> GHMQGQIIHHRNFQSQFDTTGNTLYNNAWVCSLNVIKSRDGNNYSALEDITSDNQAFNNILEGIDIIECENLLKEMNVQKIPESSLFTNIKEALQAEVFNST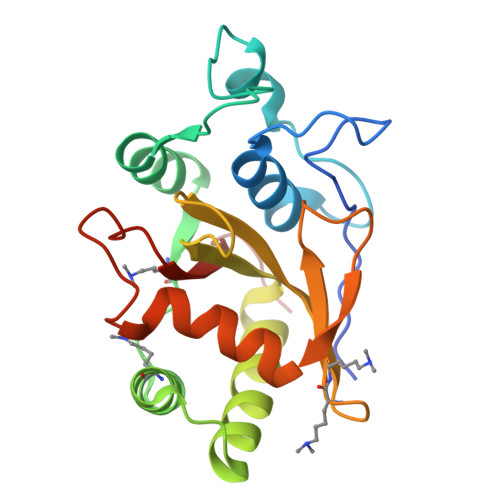VEDDFESFISYELQNHGPLMLIRPSLGSECLHAECIVGYDSEVKKVLIYDSMNTSPEWQSNIDVYDKLTLAFNDKYKNEDCSICGLYYDGVYEPK> GAMADTTEATPAAAPVAARGGELTQSTHLTLEAATKAARAAVEAAEKDGRHVSVAVVDRNGNTLVTLRGDGAGPQSYDSADRKAFTAVSWNAPTSELAKRLAQ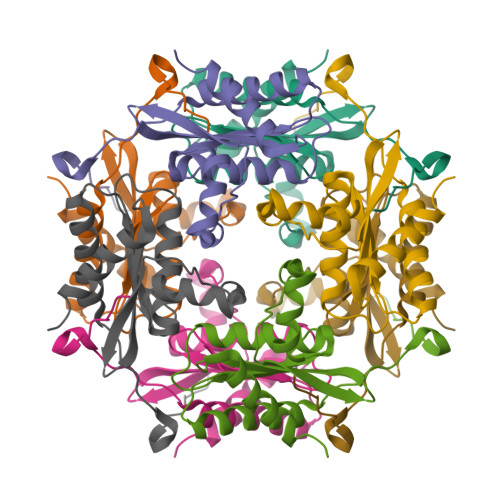APTLKDIPGTLFLAGGTPVTAKGAPVAGIGVAGAPSGDLDEQYARAGAAVLGH>[2x]HTHWGYTGHDSPESWGNLSEEFRLC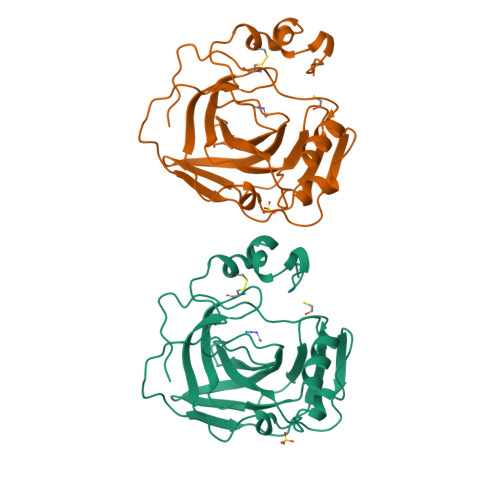STGKNQSPVNITETVSGKLPAIKVNYKPSMVDVENNGHTIQVNYPEGGNTLTVNGRTYTLKQFHFHVPSENQIKGRTFPMEAHFVHLDENKQPLVLAVLYEAGKTNGRLSSIWNVMPMTAGKVKLNQPFDASTLLPKRLKYYRFAGSLTTPPCTEGVSWLVLKTYDHIDQAQAEKFTRAVGSENNRPVQPLNARVVIE> GSADINIFSVASGHLYERMLNIMMVSVMKHTKHSVKFWFIEQFLSPSFKKFLPHLAKEYGFSYEMVTYKWPHWLRGQREKQREIWGYKILFLDVLFPLSLDKVIFVDADQIVRTDMYDLVQLDLEGAPYGFTPMCDSRKEMEGFRFWKQGYWKSHLRGRPYHISALYVVDLNRFRALAAGDRLRGQYHTLSADPNSLANLDQDLPNNMQAMIPIKSLPQEWLWCETWCADEDLKTAR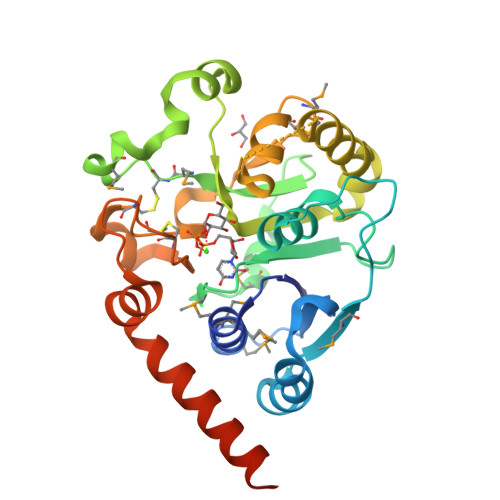TIDLCNNPLTKEPKLDRARRQVPEWTEYDNEIAELAVRVRAASKQSRREEDEKKDV>HTSPLLAPVRQIHAFGDSYSDNGESQRLTREMLAKGIAGAQALPGEVYWQGRWSNGPTAVEVLA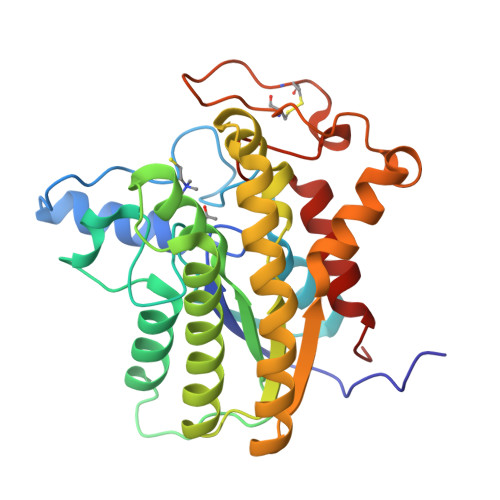RQLGAQLADHAVGGAKSGADNYYGWMSAYRHTGLAGQVDAYLATLDGKPVDGQALHFIFVSANDFFEHEDFAGEQPLEQLAGSSVANIRAAVQRLGEAGARRFLVVSSTDLSVVPAVVAGNRVERAQRYLQAVNASLPIQLAALRKTRGLELSWFDHLTFSRHLRRNPARYGLVELDAPCQPTQPSVRPACANPDQYYFWNEWHPTRRVHQLAGEAMAARYAR[2x]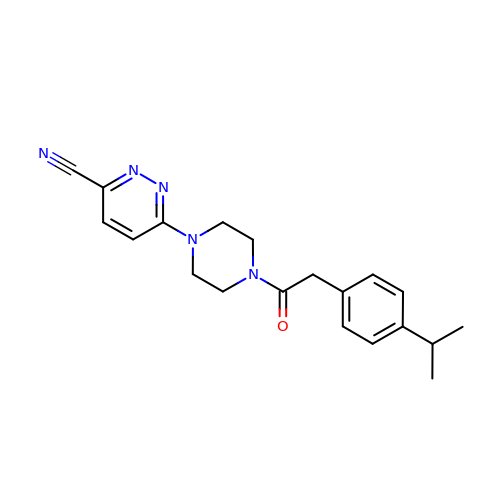6-(4-{[4-(propan-2-yl)phenyl]acetyl}piperazin-1-yl)pyridazine-3-carbonitrile | C20 H23 N5 O | LGWDVWIZDPGCFG-UHFFFAOYSA-N The loading of ring-shaped, replicative helicases onto DNA constitutes a key event during the initiation of chromosomal DNA replication. In Orc1–5, the AAA+ modules are augmented by a C-terminal HTH domain of the winged-helix (WH) type and co-assemble into a pentameric ring that can exist in both open (active) or closed (autoinhibited) configurations. Structural studies have revealed that the initiator binds DNA in the center of the ORC ring, bending DNA to prepare origins for Mcm2–7 recruitment and loading. To resolve these outstanding questions, we determined cryo-EM structures of DNA-bound Drosophila ORC (DmORC) assemblies in the presence and absence of the co-loader Cdc6.

In the DNA-bound initiator·co-loader complex, DmORC and DmCdc6 form a two-tiered hexameric ring, with each layer comprising the Orc1–5/Cdc6 AAA+ ATPase and WH domains, respectively. In the Drosophila complex, both tiers are planar and oriented perpendicular to the DNA axis within ORC’s central channel. The co-loader Cdc6 is phylogenetically most closely related to ORC’s Orc1 subunit15 and adopts a similar 3D structure as Orc1 in the ternary initiator·co-loader complex. In DmORC·DNA·Cdc6, the co-loader occupies the position between Orc1 and Orc2 and engages in canonical and non-canonical AAA+/AAA+ interactions with Orc1 and Orc2, respectively, to close the ORC ring. The N-terminus of Orc3, part of which folds into a β-strand that abuts the central β-sheet of the Orc2 AAA+ core, is sandwiched in between the Orc2 and Cdc6 AAA+ domains, sealing the ATPase ring and forming a tripartite interface. Two conserved Cdc6 arginines positioned in a helix that typically harbors the arginine finger in AAA+ ATPases—a residue involved in stimulating ATP hydrolysis of the adjacent protomer—contribute to the interaction network, indicating that this region in Cdc6 has been co-opted to mediate protein-protein interactions at the non-catalytic Orc2/Cdc6 site.

> SNAPRRSIHLSNIVEQRVFEDDEIISTPKRGRSKKTVQDNDEDYSPKKSVQKTPTRTRRSSTTTKTATTPSKGITTATATPMTPSQKMKKIRAGELSPSMQQRTDLPAKDSSKSELQLAREQLHVSVVPKSLPCREREFENIYAFLEGKIQDQCGGCMYVSGVPGTGKTATVTGVIRTLQRMAKQNELPAFEYLEINGMRLTEPRQAYVQIYKQLTGKTVSWEQAHALLEKRFTTPAPRRVTTVLLVDELDILCNRRQDVVYNLLDWPTKSAAKLVVVTIANTMDLPERLLMGKVTSRLGLTRLTFQPYSHKQLQEIVTARLGGSETFKGEAVQLVARKVAAVSGDARRALDICRRATEIADTAAVKCVTMLHVQQALAEMIASAKVQAIRNCSRMEQIFLQAIAAEVTRTGVEETTFMGVYQQVETIAAFMGVTFPPPGRALRLCSKLGAERLIISEHSRNDLFQKILLNVSADDIHYALRVEEMVN;> MSASNKGGYKTPRKENLMSIENLTNSEEESEDLNTAMVGNAVESQPKVTSRRSTRRPSPTKKYQAYQKESNGKGQEERIVVNYVEMSDERSSDAEDQEEEESIEESENAARPAAKDLHLIQSEYNVAGTSMFGFNTPKKRDAMALAALNATPCTPKTPKTPRLGVKTPDTKRKKSMDQPKTPAHVRTRVKKQIAKIVADSDEDFSGDESDFRPSDEESSSSSSSSDAGNSSDNDAADDEPKTPSRARRAIVVPVLPKTPSAARLRQSARAKKSNEFVPESDGYFHSHASSKILTSDHTLDRLKNPRLAADRVFSLLSEIKTSAEHEGSINAIMEEYRSYFPKWMCILNEGFNILLYGLGSKHQLLQSFHREVLHKQTVLVVNGFFPSLTIKDMLDSITSDILDAGISPANPHEAVDMIEEEFALIPETHLFLIVHNLDGAMLRNVKAQAILSRLARIPNIHLLASIDHINTPLLWDQGKLCSFNFSWWDCTTMLPYTNETAFENSLLVQNSGELALSSMRSVFSSLTTNSRGIYMLIVKYQLKNKGNATYQGMPFRDLYSSCREAFLVSSDLALRAQLTEFLDHKLVKSKRSVDGSEQLTIPIDGALLQQFLEEQEKK;> MDPTISVSKGCFVYKNGATRAGKKAASKRKRPAAESSSLLGKEVVQQPFYEEYRKAWNQINDHIADLQHRSYARTLEQLVDFVVGQAERDTPDEVLPTAALLTGINQPDHLSQFTALTQRLHAQRAAMVCVLQSRDCATLKAAVETLVFGLVEDNAEVEQMEDEDEDEDGAERDRKRLRRSQCTMKQLKSWYTNNFDSEQKRRQLVVILPDFECFNASVLQDLILILSAHCGSLPFVLVLGVATAMTAVHGTLPYHVSSKIRLRVFQTQAAPTGLNEVLDKVLLSPKYAFHLSGKTFKFLTHIFLYYDFSIHGFIQGFKYCLMEHFFGGNAFALCTDYSKALGRIKQLTHEDMETIRRLPSFRPYVEQINDCKRIIAVLTDDDYLKKKLPQLLRDCLLHFLLFRCSLEFLTELVGDLPRCPLGKLRRELYVNCLNRAIISTPEYKECLQMLSFLSKDEFVAKVNRALERTEQFLVEEIAPLELGEACTAVLRPKLEAIRLAVDEVVKATMATITTTSPNETRQATDHLTPVASRQELKDQLLQRSKEDKMRHQLNTPTTQFGRALQKTLQLIETQIVQDHLRALQDAPPIHELFVFSDIATVRRNIIGAPRAALHTALNNPHFYMQCKCCELQDQSLLVGTLPDLSVVYKLHLECGRMINLFDWLQAFRSVVSDSDHEEVAQEQIDPQIQARFTRAVAELQFLGYIKMSKRKTDHATRLTW;> SNAMPEADRELVSIRRFLKERLQRDYTTLRGYAKERSNVRLLLQRTAEMGESNSLLLLGPRGSGKTTLINSVLADLLPNKSFGENTLIVHLDGNLHTDDRVALKSITVQMQLENAADGKVFGSFAENLAFLLQCLKAGGKHSKSVIFILEEFDLFCAHHNQTLLYNLFDVSQSAQAPICVLGVTCRLDVIELLEKRVKSRFSHRQVFLFPSLRRFEDYVDLCRDLLSLPTGNSLLLAAEKIYNLQNIQSGALYFSRNHFDPGEYGFSPRLRDAWNKQICKVLATQQARSTLQALHDFDISEAYLKNFLFRLVAHLRPQSPHITAEKMAAVGSQFEGDDKIELLCGLSVLELCLIIAIKHHSQIYDRDSFNFEIIYARFSKFAKVSTTMQAVERSIVLKAFEHLRIAELIMPLTGGAGGGVGKVQKEFEMHKLALTYSQIHHCMQRYQALPTEVAQWAQSSLI;> MEAICSSLEPLFPCREAAIETLGELIGDSSETYPSAIYLFGHSGTGKTALTRAFLKECGKRQNVRTAHLNAIECYTTKIMLEILLDSLAPDQGDALKVDNMLDFVEQLRRQAATRVEDQGFLIAVDNAERLRDMDANVLPVLLRLQELTNLNLCVILLSQLPFEKFYNKTGLSEIVCLHLAQYNKAETQRILGSDFQQVRNQLLEQFAQDKKRLEICQEAVTEDFYNNYLNLFLSVFYKACRDVPELQLTARKCLSTYLEPVLDGTVDATDISRLWRHIAGPLRSALTQIYMRIEKPAEEVEDFTAIEDQSVRKLAQSLELPYYAKFLLIAAFLASHNAAKQDKRLFVKHHGKQRKRMQTVNARAKTTEKMSTTLGPKSFSIDRLLAIFYAILEEKVGLTCNLLSQISTLVHLNLLSFVSGEQNIMEGSARLQCTIGLEFVLQIGKVVGFNVRQYLCDFM;> MTTLIEQLITKMGLREEPNVLEKTTELVRLLELRSTNVPLQINEYGKIVLCADLASCMIGIAFDKEQALKLSGLRKSQYLNNKRMFEKLLDLNKLASVNDICVQLGLNEVARKAEELMTLFKGVAATEDMGTDTSHPQYATMAVFQACRLLKKKVSKSKLMPFSNLRPSQFQLLEQQWERMIAKHHKESKVPSSTDMEGKLKENQNENIKGHEAKKAHKPPPEDYEIWKARMLAKAQAKLKELEASQSHMDSQLLEA;> SNANNLPSPSRNKYQNARRVLNSAETQNLPGRESQLQELREFFSNHLESQTSGSLYVSGQPGTGKTACLSLLLRDPDFSKRLQRVYINCTSIASVGAVYKKLCTELQLKVSGRTERDHLEAIQRHLKTAKRMLLLVLDEIDQLCTSRQEVLYTIFEWPALPGSRILLVGIANSLDLTDRALMRLNARCELKPRLMHFPPYSKQQIVEIFKSRLAEAEVLDVFPPVTLQLLAAKVSAISGDVRRALDIGRRVVEIAEQQKRDGEKEFNMKALQLEGKDAVEAKEKQDTLKPVQVTQVAAVLNKVYGASQNLEEDIEASFPLQQKLMLCTLVLMLRNERNKDISMGRLHEVYRRVCAKRNILALDQAEFTGTVDLVETRGILRIMRKKEPRLHKVLLQWDEEEVHAALSDKQLIASILSDTACLSK>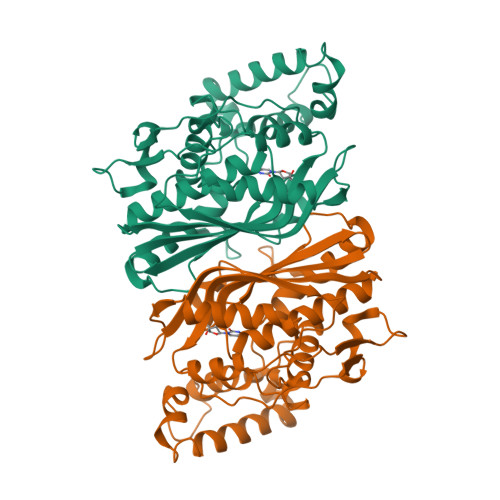 MLEQPYLDLAKKVLDEGHFKPDRTHTGTYSIFGHQMRFDLSKGFPLLTTKKVPFGLIKSELLWFLHGDTNIRFLLQHRNHIWDEWAFEKWVKSDEYHGPDMTDFGHRSQKDPEFAAVYHEEMAKFDDRVLHDDAFAAKYGDLGLVYGSQWRAWHTSKGDTIDQLGDVIEQIKTHPYSRRLIVSAWNPEDVPTMALPPCHTLYQFYVNDGKLSLQLYQRSADIFLGVPFNIASYALLTHLVAHECGLEVGEFIHTFGDAHLAVNHLDQIKEQLSRTPRPAPTLQLNPDKHDIFDFDMKDIKLLNYDPYPAIKAPVAV>MELYLDTSDVVAVKALSRIFPLAGVTTNPSIIAAGKKPLDVVLPQLHEAMGGQGRLFAQVMATTAEGMVNDALKLRSIIADIVVXVPVTAEGLAAIKMLKAEGIPTCGTAVYGAAQGLLSALAGAEYVGPYVNVIDAQGGSGIQTVTDLHQLLKMHAPQAKVCAAGFKTPRQALDCLLAGCESITLPLDVAQQMISYPAVDAAVAKFEQDWQGAFGRTSITSHH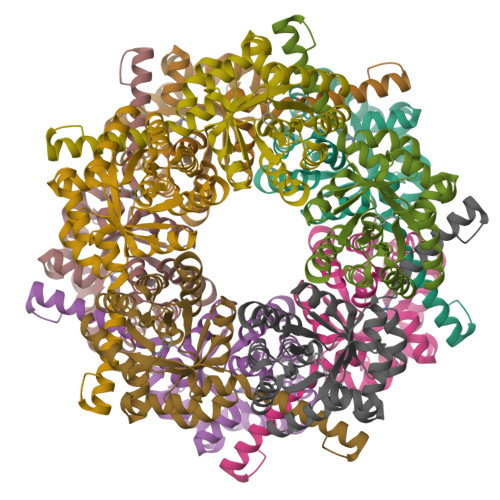HHH[10x]> MATYSLANERLRALEDIEREIGAILQNAGTVILELSKEKTNERLLDRQAAAFTASVQHVEAELSAQIR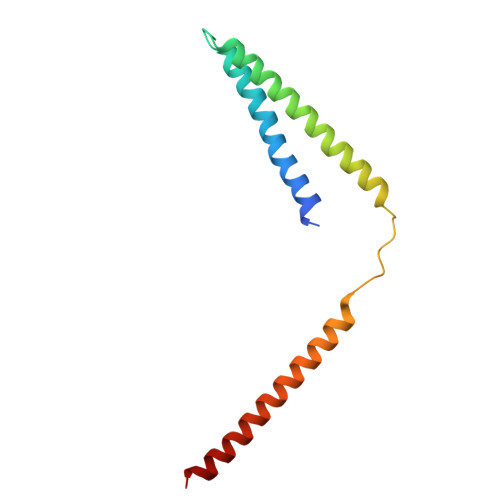YLTQVATGQPHEGSSYSSRKDCQMALKRVDYARLKLSDVARTCEQMLEN> MELKEESFRDPAEVLGTG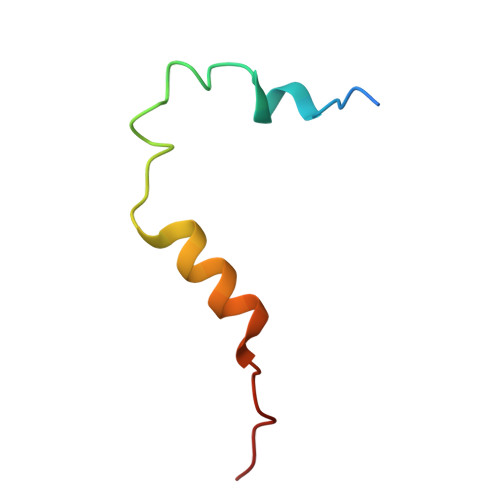AEVDYLEQFGTSSFKESALRKQSLYLKF>VSPKTYKDADFYVAPTQQDVNYDLVDDFGANGNDTSDDSNALQRAINAISRKPNGGTLLIPNGTYHFLGIQMKSNVHIRVESDVIIKPTWNGDGKNHRLFEVGVNNIVRNFSFQGLGNGFLVDFKDSRDKNLAVFKLGDVRNYKISNFTIDDNKTIFASILVDVTERNGRLHWSRNGIIERIKQNNALFGYGLIQTYGADNILFRNLHSEGGIALRMETDNLLMKNYKQGGIRNIFADNIRCSKGLAAVMFGPHFMKNGDVQVTNVSSVSCGSAVRSDSGFVELFSPTDEVHTRQSWKQAVESKLGRGCAQTPYARGNGGTRWAARVTQK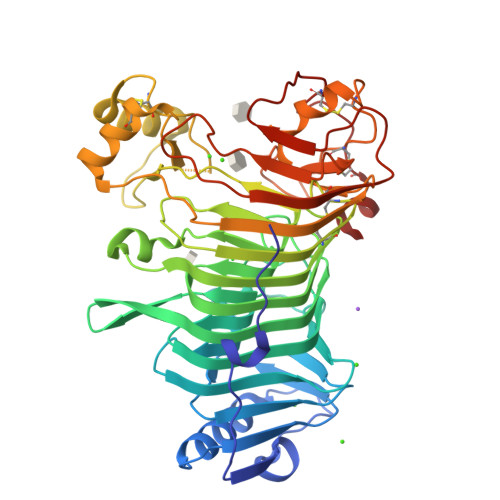DACLDKAKLEYGIEPGSFGTVKVFDVTARFGYNADLKQDQLDYFSTSNPMCKRVCLPTKEQWSKQGQIYIGPSLAAVIDTTPETSKYDYDVKTFNVKRINFPVNSHKTIDTNTESSRVCNYYGMSECSSSRWER[2x]>[4x]MDFLDSLIWERVVDDQYVTNPTFCISDYFEIVRQPGDGNCFYHSIAELFFDVKTPFSFRKVKEHLRLAADAFYDTEPEAIGTGVTKEEYIQAAMKDNEWGGSLEASMLSKQLQITIILWVVNQTEQVTAAIKFGPGRVSTALNLMHVGRTHFDALRVINQLEDNQLQSRSGSHHHHHH;>MATLNILVRNDKGRSSSYEV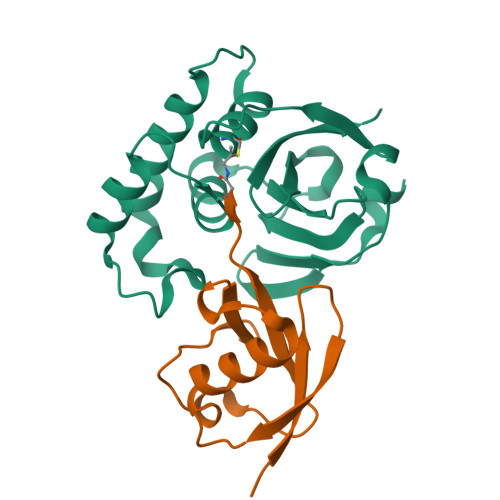QLTQTVAVLKQQVCQRERVQADQFWLSFEGKPMDDEHPLGEYGLTTGCTVFMNLRLRG[4x]> MAAVVKSVALAGRPTTPDRVHEVLGRSMLVDGLDIVLDLTRSGGSYLVDAITGRRYLDMFTFVASSALGMNPPALVDDREFHAELMQAALNKPSNSDVYSVAMARFVETFARVLGDPALPHLFFVEGGALAVENALKAAFDWKSRHNQAHGIDPALGTQVLHLRGAFHGRSGYTLSLTNTKPTITARFPKFDWPRIDAPYMRPGLDEPAMAALEAEALRQARAAFETRPHDIACFVAEPIQGEGGDRHFRPEFFAAMRELCDEFDALLIFDEVQT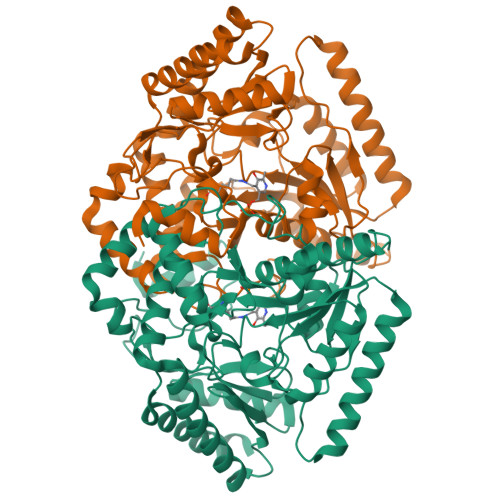GCGLTGTAWAYQQLDVAPDIVAFGKKTQVCGVMAGRRVDEVADNVFAVPSRLNSSWGGNLTDMVRARRILEVIEAEGLFERAVQHGKYLRARLDELAADFPAVVLDPRGRGLMCAFSLPTTADRDELIRQLWQRAVIVLPAGADTVRFRPPLTVSTAEIDAAIAAVRSALPVVT The regulator of telomere elongation helicase 1 (RTEL1) is an Fe-S cluster and DEAH motif-containing DNA helicase with ATP-dependent 5′ to 3′ helicase activity. RTEL1 plays essential roles in telomere maintenance, DNA repair, meiotic recombination, and genome-wide replication. It is a modular protein consisting of an N-terminal helicase domain followed by two tandem harmonin homology domains 1&2 (HHD1 and HHD2), a PCNA-interacting protein-box (PIP-box) motif, and a C-terminal C4C4 type RING domain. RTEL1 is an anti-recombinase and executes non-crossovers by promoting the synthesis-dependent strand annealing (SDSA) pathway of homologous recombination through disassembling displacement-loop (D-loop) intermediates during the DNA repair and meiotic recombination processes.

To understand the structural basis of RPA 32C and RTEL1 HHD2 interaction, we determined the structure of HHD2 at a resolution of 1.6 Å using X-ray crystallography (details in the Materials and Methods section). The structure revealed that HHD2 consists of five helices, from H1 to H5, connected by a short loop. All the helices are mainly α-helical (3.613 helix) except the N- and C-termini of H4 and the N-terminal of H5, which consists of short 310 helices. The overall topology of RTEL1 HHD2 is similar to the N-terminal domain of the human Harmonin. A sequence alignment of HHD2 corresponding sequences of RTEL1 across the vertebrates, showed that the evolutionarily conserved residues are mainly present in the core region stabilizing the tertiary structure. The electrostatic surface potential of HHD2 revealed a distinct pattern of positively and negatively charged opposite surfaces. RPA 32C binds mainly to the solvent-exposed surfaces of helix H1 and H2, while DNA binds in the pocket formed by helix H1, H2, and H4, suggesting HHD2 adapts to bind DNA and 32C on the same surface. The electrostatic surface potential analysis, in combination with NMR CSPs, revealed that the positively charged surface of HHD2 could interacts with the negatively charged surface of 32C. Using NMR spectroscopy and isothermal titration calorimetry (ITC), we showed that HHD2 also interacts with DNA using the RPA 32C binding surface. This study establishes HHD2 as a novel accessory domain of RTEL1 that mediates both protein–protein and protein–DNA interactions. The X-ray crystal structure of the HHD2 domain of RTEL1 reported here is the first structure of any domains of RTEL1.

>[7x]MGSSHHHHHHSGQHAVSAYLADARRALGSAGCSQLLAALTAYKQDDDLDKVLAVLAALTTAKPEDFPLLHRFSMFVRPHHKQRFSQTCTDLTGRPY>[2x]HHHHHHKICIGTKSRLSVPSNKEHHYRNLRDRYTNCTYVDGNLELTWLPNENLDLSFLDNIREVTGYILISHVDVKKVVFPKLQIIRGRTLFSLSVEEEKYALFVTYSKMYTLEIPDLRDVLNGQVGFHNNYNLCHMRTIQWSEIVSNGTDAYYNYDFTAPERECPKCHESCTHGCWGEGPKNCQKFSKLTCSPQCAGGRCYGPKPRECCHLFCAGGCTGPTQKDCIACKNFFDEGVCKEECPPMRKYNPTTYVLETNPEGKYAYGATCVKECPGHLLRDNGACVRSCPQDKMDKGGECVPCNGPCPKTCPG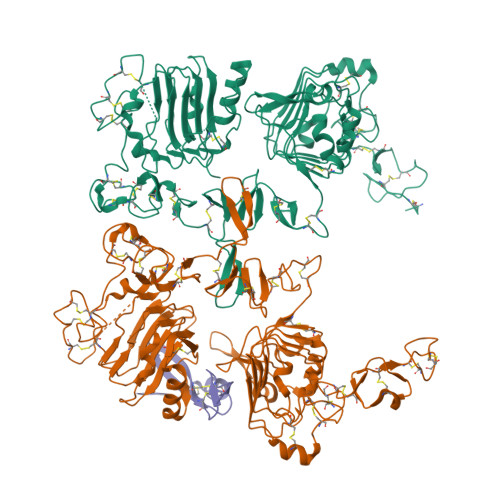VTVLHAGNIDSFRNCTVIDGNIRILDQTFSGFQDVYANYTMGPRYIPLDPERLEVFSTVKEITGYLNIEGTHPQFRNLSYFRNLETIHGRQLMESMFAALAIVKSSLYSLEMRNLKQISSGSVVIQHNRDLCYVSNIRWPAIQKEPEQKVWVNENLRADLCEKNGTICSDQCNEDGCWGAGTDQCLNCKNFNFNGTCIADCGYISNAYKFDNRTCKICHPECRTCNGAGADHCQECVHVRDGQHCVSECPKNKYNDRGVCRECHATCDGCTGPKDTIGIGACTHHHHHH;> TFPTYKCPETFDAWYCLNDAHCFAVKIADLPVYSCECAIGFMGQRCEYKEID> MSRKQLALFEPTLVVQALKEAVKKLNPQAQWRNPVMFIVWIGSLLTTCISIAMASGAMPGNALFSAAISGWLWITVLFANFAEALAEGRSKAQANSLKGVKKTAFARKLREPKYGAAADKVPADQLRKGDIVLVEAGDIIPCDGEVIEGGASVDESAITGESAPVIRESGGDFASVTGGTRILSDWLVIECSVNPGETFLDRMIAMVEGAQRRKTPNEIALTILLIALTIVFLLATATLWPFSAWGGNAVSVTVLVALLVCLIPTTIGGLLSAIGVAGMSRMLGANVIATSGRAVEAAGDVDVLLLNKTGTITLGNRQASEFIPAQGVDEKTLADAAQLASLADETPEGRSIVILAKQRFNLRERDVQSLHATFVPFTAQSRMSGINIDNRMIRKGSVDAIRRHVEANGGHFPTDVDQKVDQVARQGATPLVVVEGSRVLGVI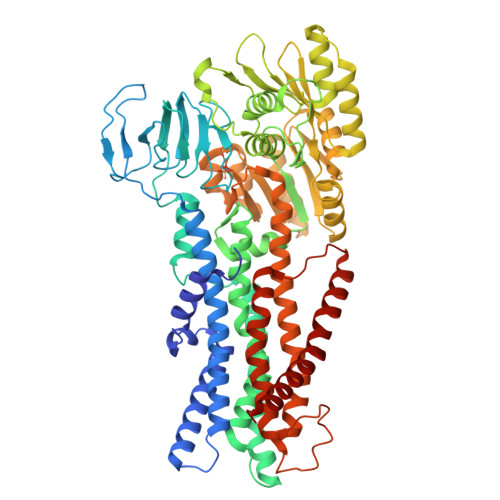ALKDIVKGGIKERFAQLRKMGIKTVMITGDNRLTAAAIAAEAGVDDFLAEATPEAKLALIRQYQAEGRLVAMTGDGTNDAPALAQADVAVAMNSGTQAAKEAGNMVDLDSNPTKLIEVVHIGKQMLMTRGSLTTFSIANDVAKYFAIIPAAFAATYPQLNALNIMCLHSPDSAILSAVIFNALIIVFLIPLALKGVSYKPLTASAMLRRNLWIYGLGGLLVPFIGIKVIDLLLTVCGLV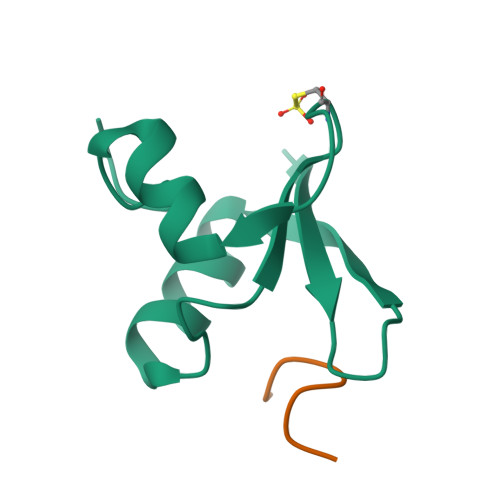>[2x]GPLESHGAARKWFYKDPQGEIQGPFTTQEMAEWFQAGYFSMSLLVKRGCDEGFQPLGEVIKMWGRVPFAPGPS;>[2x]GPLGSAPTRPPPGLTN One of the most prominent GDHs capable of DET is the bacteria-derived FADGDH complex, with the first reported example derived from Burkholderia cepacia (BcGDH). Bacteria-derived FADGDH complexes are composed of three distinct subunits: a catalytic subunit harboring an FAD cofactor in its catalytic center with an iron sulfur cluster (Fe-S; 3Fe-4S) as the primary electron acceptor of FAD, a small subunit which is a hitch-hiker protein necessary for the bacterial TAT secretion system, and an electron transfer subunit harboring three heme c units. This enzyme can transfer electrons liberated from glucose oxidation directly to the electrode without any redox mediator as a consequence of the architecture of the electron transfer subunit. The electron transfer subunit is required for DET, and followingly, the dissociation of the electron transfer subunit eliminates BcGDH’s DET ability.

The proposed structure is modeled based on X-ray diffraction data analyses of the BcGDH complex crystal grown using the crystallization facility of JAXA on board the Japanese Experiment Module Kibo on the ISS. Through electron density analysis, a partial structure of the electron transfer subunit from βLeu314 to the C-terminal end colored in pink was determined, containing the third heme c. The overall structure revealed the third heme c region of the electron transfer subunit interacts with both catalytic and small subunits. The thioether end of the third heme c is oriented to the Fe-S cluster, and the region from βCys334 to βThr358, colored with magenta including the heme binding motif, interacts with the small subunit colored with cyan. This region is close to the intrinsic disulfide bond formed between αC213 and γC152. The catalytic subunit colored with green mainly interacts with the region between helix1 and helix2 and includes the colored-region in magenta (βIle384 to βAsn394), where the sixth ligand (βM386) of the third heme is located. The edge-to-edge distance between the third heme c and the 3Fe-4S in the catalytic subunit is 7~8 Å. Because of this short distance, it is expected electrons are directly transferred between the 3Fe-4S of the catalytic subunit to the third heme c in the electron transfer subunit. Based on the structural model, 14 candidate amino acid residues were selected to form disulfide bond pairs between the small and electron transfer subunits (5 pairs), as well as the catalytic and electron transfer subunits (9 pairs).

> MADTDTQKADVVVVGSGVAGAIVAHQLAMAGKAVILLEAGPRMPRWEIVERFRNQPDKMDFMAPYPSSPWAPHPEYGPPNDYLILKGEHKFNSQYIRAVGGTTWHWAASAWRFIPNDFKMKSVYGVGRDWPIQYDDLEPYYQRAEEELGVWGPGPEEDLYSPRKQPYPMPPLPLSFNEQTIKTALNNYDPKFHVVTEPVARNSRPYDGRPTCCGNNNCMPICPIGAMYNGIVHVEKAERAGAKLIENAVVYKLETGPDKRIVAALYKDKTGAEHRVEGKYFVLAANGIETPKILLMSANRDFPNGVANSSDMVGRNLMDHPGTGVSFYASEKLWPGRGPQEMTSLIGFRDGPFRATEAAKKIHLSNLSRIDQETQKIFKAGKLMKPDELDAQIRDRSARYVQFDCFHEILPQPENRIVPSKTATDAIGIPRPEITYAIDDYVKRGAAHTREVYATAAKVLGGTDVVFNDEFAPNNHITGSTIMGADARDSVVDKDCRTFDHPNLFISSSATMPTVGTVNVTLTIAALALRMSDTLKKEV;> MGKSTLTFLIAGCLALPGFARAADAADPALVKRGEYLATAGDCMACHTVKGGKPYAGGLGMPVPMLGKIYTSNITPDPDTGIGKWTFEDFERAVRHGVSKNGDNLYPAMPYVSYAKITDDDVRALYAYFMHGVEPVKQAPPKNEIPALLSMRWPLKIWNWLFLKDGPYQPKPSQSAEWNRGAYLVQGLAHCSTCHTPRGIAMQEKSLDETGGSFLAGSVLAGWDGYNITSDPNAGIGSWTQQQLVQYLRTGSVPGVAQAAGPMAEAVEHSFSKMTEADIGAIATYVRTVPAVADSNAKQPRSSWGKPAEDGLKLRGVALASSGIDPARLYLGNCATCHQMQGKGTPDGYYPSLFHNSTVGASNPSNLVQVILNGVQRKIGSEDIGMPAFRYDLNDAQIAALTNYVTAQFGNPAAKVTEQDVAKLRSGGPVPLLVRVRPLMLPGAVVVVLIALLGVAFWWRRRQRTPLANPPQGKAGHHHHHH;> DNPGTAPLDTFMTLSESLTGKKGLSRVIGERLLQALQKGSFKTADSLPQLAGALASGSLTPEQESLALTILEAWYLGIVDNVVITYEEALMFGVVSDTLVIRSYCPNKPGFWADKPIERQA>[2x]MNVSIEEFTHFDFQLVPEPSPLDLVITESLKNHIEVNGVKSGALLPLPFQTGIGKTYTALNFLLQQMLEQVRSELKEENTGKKSKRLLYYVTDSVDNVVSAKADLLKLIEKQTVKGEPRFTLEQQEYLKAQIVHLPNQSEQLLQCSDAVLNDVLIGFNLNAERDVQAEWSAISGLRRHASNPEVKISLNRQAGYFYRNLIDRLQKKQKGADRVLLSGSLLASVETLLPGEKIRNGSAHVAFLTTSKFLKGFHNTRSRYSPLRDLSGAVLIIDEIDKQNQVILSELCKQQAQDLIWAIRTLRANFRDHQLESSPRYDKIEDLFEPLRERLEEFGTNWNLAFAFNTEGANLNERPV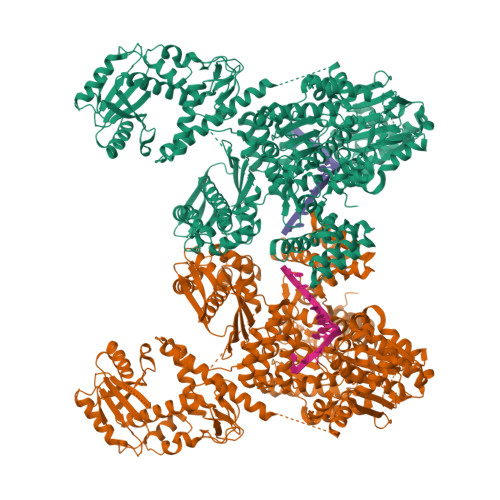RLFSDRSFTHVSSATHKLSLKSDFLRRKNLIFSDEKVEGSLIEKHGLLTRFVNEADVIYQWFLGTMRKAVFQYWENVRGLEIEVRENRSLEGTFQEAVQSLLTHFNLQEFESAVYESFDTRGLRQSAGGKANKLSSSKSYHHTGLKLVEVAHNQGTRDTVNCKASFLNTSPSGVLADMVDAGAVILGISATARADTVIHNFDFKYLNERLGNKLLSLSREQKQRVNNYYHSRRNYKDNGVVLTVKYLNSRDAFLDALLEEYKPEARSSHFILNHYLGIAESEQAFVRSWLSKLLASIKAFISSPDNRYMLSLLNRTLDTTRQNINDFIQFCCDKWAKEFNVKTKTFFGVNADWMRLVGYDEISKHLNTELGKVVVFSTYASMGAGKNPDYAVNLALEGESLISVADVTYSTQLRSDIDSIYLEKPTQLLLSDDYSHTANQLCQFHQILSLQENGELSPKSAENWCRQQLMGMSRERSLQQYHQTSDYQSAVRKYIEQAVGRAGRTSLKRKQILLFVDSGLKEILAEESRDPSLFSHEYVALVNKAKSAGKSIVEDRAVRRLFNLAQRNNKDGMLSIKALVHRLHNQPASKSDIQEWQDIRTQLLRYPTVAFQPERFNRLYLQSMTKGYYRYQGNLDGDPNSFEFFDRVPYGDMVSEEDCSLATLVQNQYVRPWFERKGFACSWQKEANVMTPIMFTNIYKGALGEQAVEAVLTAFDFTFEEVPNSIYERFDNRVIFAGIEQPIWLDSKYWKHEGNESSEGYSSKIALVEEEFGPSKFIYVNALGDTSKPIRYLNSCFVETSPQLAKVIEIPALIDDSNADTNRTAVQELIKWLHHS>[2x]MGSSHHHHHHSSGENLYFQGHMSNTSWRKSEVLAVPLQPTLQQEVILARMEQILASRALTDDERAQLLYERGVLYDSLGLRALARNDFSQALAIRPDMPEVFNYLGIYLTQAGNFDAAYEAFDSVLELDPTYNYAHLNRGIALYYGGRDKLAQDDLLAFYQDDPNDPFRSLWLYLAEQKLDEKQAKEVLKQHFEKSDKEQWGWNIVEFYLGNISEQTLMERLKADATDNTSLAEHLSETNFYLGKYYLSLGDLDSATALFKLAVANNVHNFVEHRYALLELSLLGQDQDDLAESDQQ;>[2x]MNMFFRLTALAGLLAIAGQTFAVEDITRADQIPVLKEETQHATVSERVTSRFTRSHYRQFDLDQAFSAKIFDRYLNLLDYSHNVLLASDVEQFAKKKTELGDELRSGKLDVFYDLYNLAQKRRFERYQYALSVLEKPMDFTGNDTYNLDRSKAPWPKNEAELNALWDSKVKFDELSLKLTGKTDKEIRETLTRRYKFAIRRLAQTNSEDVFSLAMTAFAREIDPHTNYLSPRNTEQFNTEMSLSLEGIGAVLQMDDDYTVINSMVAGGPAAKSKAISVGDKIVGVGQTGK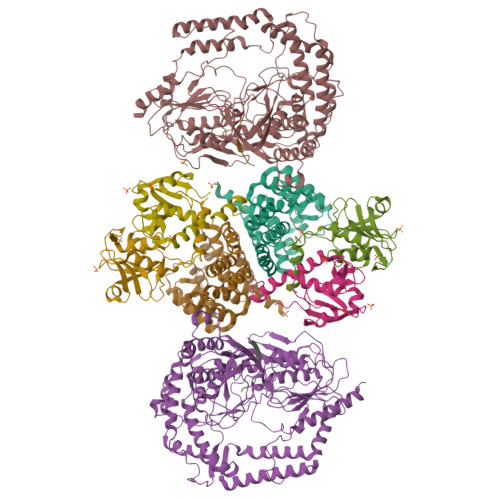PMVDVIGWRLDDVVALIKGPKGSKVRLEILPAGKGTKTRTVTLTRERIRLEDRAVKMSVKTVGKEKVGVLDIPGFYVGLTDDVKVQLQKLEKQNVSSVIIDLRSNGGGALTEAVSLSGLFIPAGPIVQVRDNNGKVREDSDTDGQVFYKGPLVVLVDRFSAAASEIFAAAMQDYGRALVVGEPTFGAGTVQQYRSLNRIYDQMLRPEWPALGSVQYTIQKFYRVNGGSTQRKGVTPDIIMPTGNEETETGEKFEDNALPWDSIDAATYVKSGDLTAFEPELLKEHNARIAKDPEFQNIMKDIARFNAMKDKRNIVSLNYAVREKENNEDDATRLARLNERFKREGKPELKKLDDLPKDYQEPDPYLDETVNIALDLAKLEKARPAEQPAPVKHHHHHH;>MSANNTAKNMHPETRAVGSETSSLQASQDEFENLVRNVDVKSRIMDQYADWKGVRYRLGGSTKKGIDCSGFVQRTFREQFGLELPRSTYEQQEMGKSVSRSNLRTGDLVLFRAGSTGRHVGIYIGNNQFVHASTSSGVIISSMNEPYWKKRYNEARRVLSRSHHHHHH[4x]>SQAEFDKAAEEVKNLKTKPADDEMLF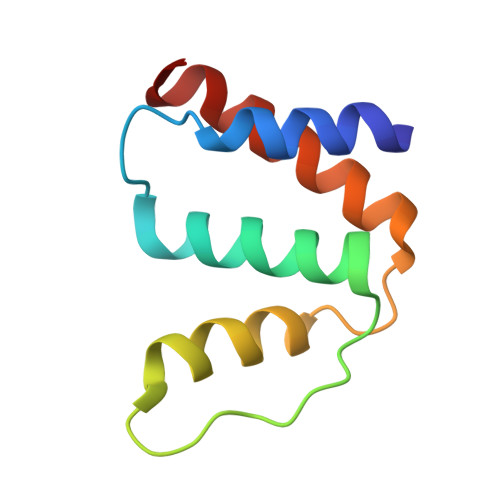IYSHYKQATVGDINTERPGMLDFKGKAKWDAWNQLKGTSKEDAMKSYIDKVEELKKKYGI[3x]> GSSTDLPKSNKNNNFITHNLHTVWIGGPLPDITKSYLKVWRDINPDYTHITWIDTDNKFVALYNNAVKELREYTLKQYLVGDSNATANDYYDQAVQIERGVRENVYLPHGNDIERIKTIKKIAGSLGDNKVQEYRTKIETIESSFVEMIDGQQGHYQHVSALFEQFSEMDNLRATALKQIYEREINDRGNLAAASDILRLVALQTQGGVYIDTDLLPHIDWDLIESTKLFLMNDNNSVERVYSKEIYLEIEKYKQLTGSKTNKIRSGLTKSQINEIQRLTEENNLFKHLNELEKNCFYSDNSVRGWTNAMLACNENNGFMNALMDRIILNYTILDEFIISNIVTDGEMLNFTEKMSAQFGLNAEHEGSFIPSLANYYKDSIVPNSPQATATLFMTGPTVLDTVIRVEEAVRRGIVKKEAIASLYTVEETFSSWSISQFYDKAAFYLDKVKFDISLNSAEEGILRDSCFDVIQQSKEQATHLPDIAIKFLESLNN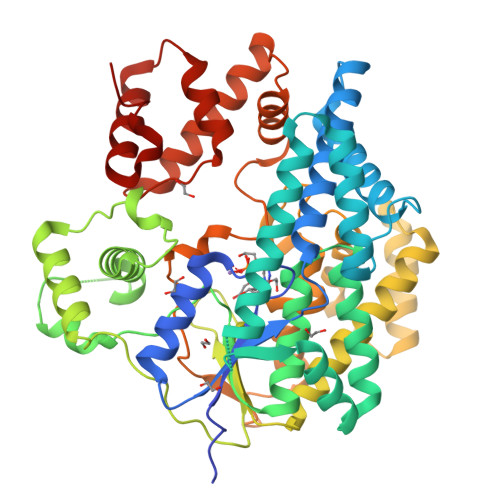FTWKQLELLIKASEFSDQYKTLATLAD5'-O-[(R)-HYDROXY(THIOPHOSPHONOOXY)PHOSPHORYL]ADENOSINE 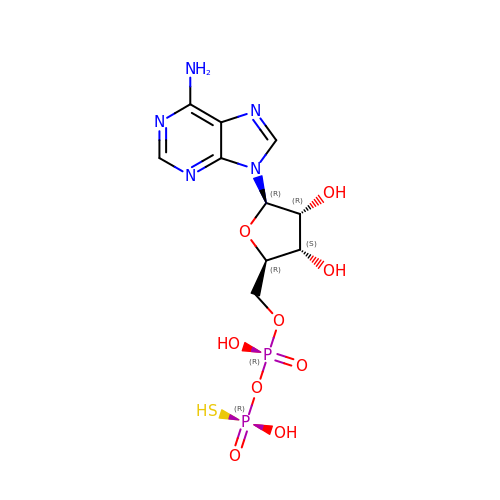| C10 H15 N5 O9 P2 S | HCIKUKNAJRJFOW-KQYNXXCUSA-N> MVSLPRMVYPQPKVLTPCRKDVLVVTPWLAPIVWEGTFNIDILNEQFRLQNTTIGLTVFAI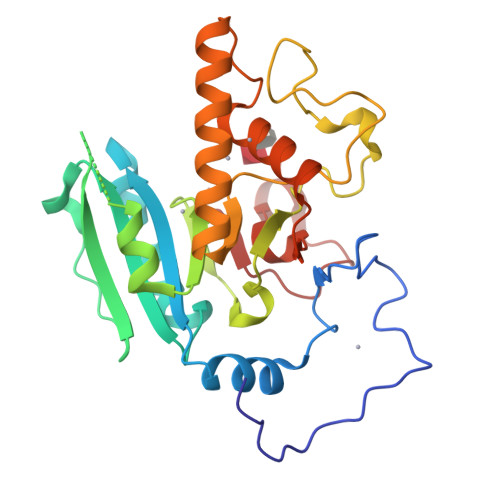KKYVAFLKLFLETAEKHFMVGHRVHYYVFTDQPAAVPRVTLGTGRQLSVLEVGAYKRWQDVSMRRMEMISDFCERRFLSEVDYLVCVDVDMEFRDHVGVEILTPLFGTLHPSFYGSSREAFTYERRPQSQAYIPKDEGDFYYMGAFFGGSVQEVQRLTRACHQAMMVDQANGIEAVWHDESHLNKYLLRHKPTKVLSPEYLWDQQLLGWPAVLRKLRFTAVP> GMDGASEIELVFRPHPTLMEKDDSAQTRYIKTSGNATVDH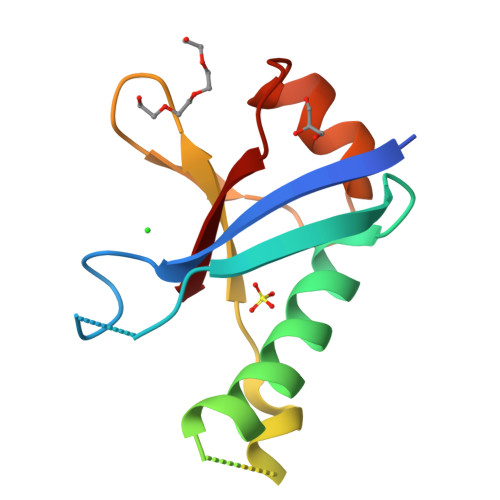LSKYLAVRLALEELRSKGESNQMNLDTASEKQYTIYIATASGQFTVLNGSFSLELVSEKYWKVNKPMELYYA>AQPPPDVEGDDCLPAYRHLFCPDLLRDKVAFITGGGSGIGFRIAEIFMRHGCHTVIASRSLPRVLTAARKLAGATGRRCLPLSMDVRAPPAVMAAVDQALKEFGRIDILINCAAGNFLCPAGALSFNAFKTVMDIDTSGTFNVSRVLYEKFFRDHGGVIVNITATLGNRGQALQVHAGSAKAAVDAMTRHLAVEWGPQNIRVNSLAPGPISGTEGLRRLGGPQASLSTKVTASPLQRLGNKTEIAHSVLYLASPLASYVTGAV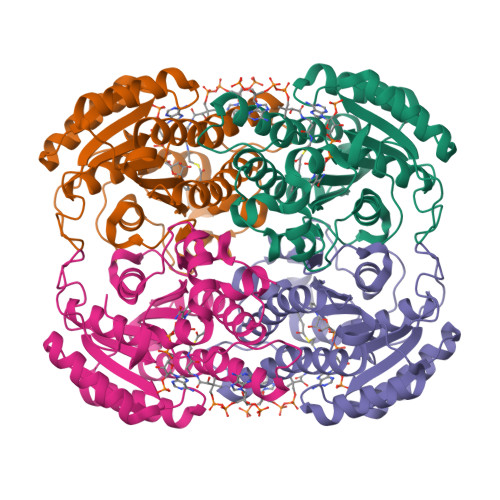LVADGGAWLTFPNG[4x]(2R)-N-[4-[2-[(4-morpholin-4-ylphenyl)amino]pyrimidin-4-yl]phenyl]pyrrolidine-2-carboxamide 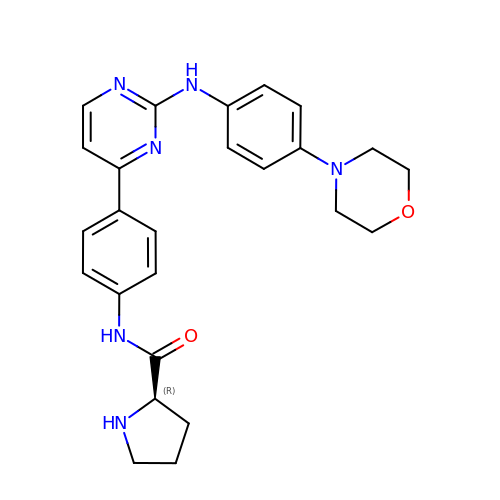| C25 H28 N6 O2 | ISOCDPQFIXDIMS-HSZRJFAPSA-N> MSESLSWMQTGDTLALSGELDQDVLLPLWEMREEAVKGITCIDLSRVSRVDT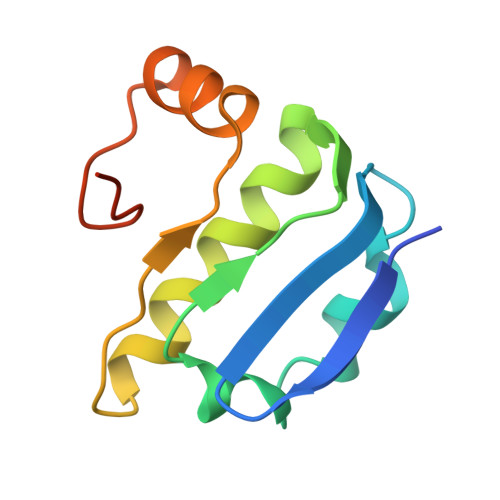GGLALLLHLIDLAKKQGNNVTLQGVNDKVYTLAKLYNLPADVLPRHHHHHHHH> MAVPFVEDWDLVQTLGEGAYGEVQLAVNRVTEEAVAVKIVDMKRAVDCPENIKKEICINKMLNHENVVKFYGHRREGNIQYLFLEYCSGGELFDRIEPDIGMPEPDAQRFFHQLMAGVVYLHGIGITHRDIKPENLLLDERDNLKISDFGLATVFRYNNRERLLNKMCGTLPYVAPELLKRREFHAEPVDVWSCGIVLTAMLAGELPWDQPSDSCQEYSDWKEKKTYLNPWKKIDSAPLALLHKILVENPSARITIPDIKKDRWYNKPLKKGAKRPRVTSGGVSESPSGHHHHHHHH

Chk1 is a key component of the DNA damage response pathway and is activated in response to intrinsic DNA damage induced by normal cellular processes such as replication fork collapse or in response to DNA damage induced by cytotoxic chemotherapeutic agents. Biochemical and genetic studies have demonstrated Chk1 to be indispensable for the S- and G2-M checkpoints. Chk1 and Chk2 negatively regulate the Cdc25 family of phosphatases thereby preventing cell cycle progression as well as directly modulating repair proteins, resulting in increased lesion repair. Chk1 inhibition, therefore, represents a novel therapeutic strategy to increase the cytotoxicity of DNA-damaging chemotherapeutic drugs in p53 pathway defective cancers.

V158411 is a novel inhibitor of the Chk1 kinase discovered through structure-based elaboration of a fragment core designed for binding at a kinase ATP-binding site. The X-ray structure of VER-154637 bound to the ATP-binding site of Chk1 showed that the two rings of the fragment were coplanar and made the expected hydrogen-bonds with the hinge motif of the kinase domain. The indolyl-pyridone core bound to Chk1 like the parent fragment, and formed the basis for subsequent molecular modeling and compound elaboration. Modeling suggested that an amide linker grafted on the pyridone position 5 would offer its carbonyl group as hydrogen-bond acceptor complementary to the hydrogen-bond donor character of the contacting water. The amide nitrogen offered the opportunity to grow towards the largely buried and structurally restrained side-chain amino group of Lys38. The X-ray structure of VER-155422 bound to Chk1 showed that the benzyl tucks underneath the flexible glycine loop, burying the apolar benzyl away from water, which presumably explains the associated affinity gain. It was then noted that reversing the intramolecular direction of the amide linker could maintain its hydrogen-bond with the conserved water, while also keeping the desired compound length for binding to Lys38. Much of the subsequent medicinal chemistry concentrated on improving the compounds physico-chemical and ADMET properties. This was done by varying substituents at the solvent-exposed 5 position of the indole ring which, from a structural point of view, can tolerate a broad range of substituents, largely unhindered from specific interactions with the protein. No attempt was made to design compounds which would be selective for Chk1 over Chk2. This led to V158411, which had the desired kinase selectivity profile and showed promising biological activity.> MDCATYATRKDKGWELNENRCVWAASVKPTSGAIMTNVGVHGKSGNAVLMTPKRRPHAQNHAGYKIKYCKQVPLIPLHGGDYILNHWETRGVDRMRIP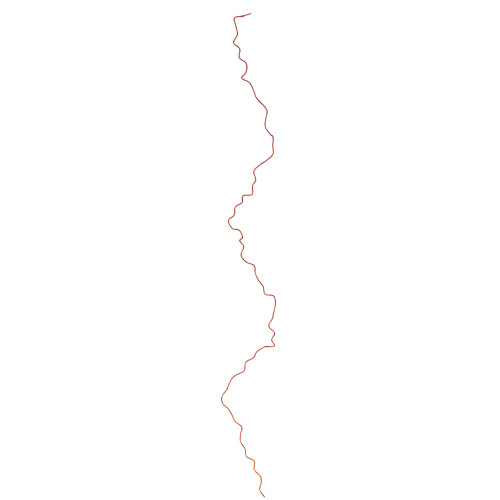GIQHAPPPPAPSGMQNAYSTHPDAYRTPLLADSHALSRMPVVQVHGPQVAPKNSHFTVAPEKHGPVEDMNAIINALPTKVDAVKLEYSASKTNRTNKRPGDGGAPPPKNLSKCHQNKLKTFARTANSGANPFRPATAAPQGLSKQPVRKPFASARNANSGANPFRPPLAHQGLSKAHVVKTAVSVANRSAGAEPFVTRNDPRALAMELANNKTISVTLGLRHWKTVSAAPPEKMSKSGVCKIATNVYNRDGGANPFLVKYEPDSLAVCPMETVEIAAVPSKRPWEGSANPRRPEQISFGMSDKPKFVNDKIGIVLRGPTLAPTLDRTATHTVTRPRALGSFHSTAGPAKHAASIMAECKDESR>GSHMQAEILLTLKLQQKLFADPRRISLLKHIALSGSISQGAKDAGISYKSAWDAINEMNQLSEHILVERATGGKGGGGAVLTRYGQRLIQLYDLLAQIQQKAFDVLSDDDALPLNSLLAAISRFSLQTSARNQWFGTITARDHDDVQQHVDVLLADGKTRLKVAITAQSGARLGLDEGKEVLILLKAPWVGITQDEAVAQNADNQLPGIISHIERGAEQCEVLMAL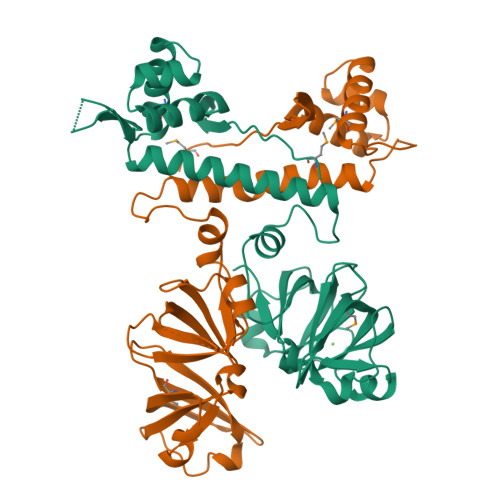PDGQTLCATVPVNEATSLQQGQNVTAYFNADSVIIATLC[2x]The cytochrome bc 1 complex, also known as respiratory complex III (CIII), in the electron-transfer chain of the inner mitochondrial membrane is a homodimer (CIII2) of two biochemically identical protomers. CIII2 catalyses the transfer of electrons from the lipophilic two-electron donor ubiquinol (QH2) to the water-soluble, one-electron acceptor protein cytochrome c, contributing to an electrochemical proton gradient across the membrane. Electron transfer within the complex occurs through the prosthetic groups of the three catalytic core subunits: heme b L and heme b H of cytochrome b (cyt b), heme c 1 of cytochrome c 1 (cyt c 1) and the [2Fe–2S] cluster of the iron–sulfur protein (ISP), often called the Rieske protein after its discoverer. The Rieske domain is tethered to the complex by one transmembrane helix and a connecting flexible linker that acts as a hinge.

(ix) +DQ+NaAsc: reduced by ascorbate and DQ. When DQ and ascorbate were added after purification (+DQ+NaAsc) density in the Qo site increased, indicating a possible low occupancy of DQ in the Qo site. The additional density was in a position similar to atovaquone. The Rieske domain was in a position in which Tyr279 and Cys189 were further apart (3.7 Å) and His190 was closer to Tyr279 (3.4 Å) compared with the ascorbate-reduced sample without added DQ. His190 was ∼2.7 Å away from the DQ density in the Qo site. The Fe–S cluster-bearing tip of the Rieske domain was well-resolved in the two ascorbate-reduced samples. Density at the hinge, where the transition from helix to random coil occurs with Pf-type inhibitors bound, and density distal to the tip was weak, indicating heterogeneity in these regions. In CIII2 with a reduced high-potential chain there was also a clear increase in density for bound quinone in Qo when DQ was added. Addition of the substrate analogue decylubiquinone to CIII2 with a reduced high-potential chain increased the occupancy of the Qo site. Under conditions that favour the enzyme–product complex we observe better density for a quinone substrate in the Qo site, which has been difficult using crystallographic studies.

>MNSLLRLPALKRGVFTMSKRGLATTVSPKTRTSNLKNGLTIASESNPLVQTATVGVWIDAGSRNENAYNNGTAHFFEHLAFKGTDKRSQHQLELDIENMGGHLNAYTSRESTVYYAKSFKDDVPKSVEILADILQHSKLAESAIDREREVITRELEEVNKQYEEVVFDHLHATAFMNQPLGRTILGPRENIQTITNTELRKFITENYTADRMVLVGAGAVDHDALVELAEKYFSHLPSSQSPVPLGTPRSSGEDANQNPIPNFVGSEVRLRDDTMPVAHIAIAVEGVSWTSEDYYTALVAQAIIGNYDRAVGTSRHQGSRLSNIVSENNLANSFQSFSTSYSDTGLWGIYLTSENTTQIDDLVHFTLKEWNRLSTSVSNLQVERAKSQLKAGLLLSLDGTTYVAEDIGRQLTTLGRRVTPAEVEAKLEAVTEHDVRAWAQKTLYDKDIALVGLGPIEGLYDYNRIRNDMSMMRW[2x];>[2x]MTRGVPRLAVAARHFSTAEAAGVKVAAQDGQSPISDLSVVLRGGSRYATVPGVSHILEKFAFQNTVPKSALRFVRELELFGGKLYTHTTREHIVLRTQFLKQDLPYFVDAFANVLKETKFQQFELTERVAPVAELDLLKRESDPAFTALEAAHEVAFRTGLGNSVYAQGYSPVTLEDVKEFARQVYAKQNVAVVGNNVVPADLQQLVGTAFADLQEGSKVTQAGTTTLHGGEARVRTSTGNALTIALPIAEPKPVYHALASFLGGPASMPWSVGASPLAQATVGTHTSVKATYHNYGDAGLFAITIKGDSPAEISQVAHKAVQALKDTGAEVTEEQAARAYAKSKFAAAEAFENPDSSASVIGMELLSGVSRIAPENVQKFTPAELSEAAAQLSASAKPVVAAVGQVHALPFADELF;>MALRKKNSLLNMANSYVLDSPQPSNLNYFWNFGSLLALCLVIQLATGITLAMHYTSHASLAFDSVEHIMRDVNFGWFIRYAHANTASFFFICIYAHMGRNIYYGSYKTPRVLPWSIGVIIFLLLIITAFMGYVLVFGQMSLWGATVICNLVSAIPWLGEDIVHFLWGGFSVGNPTLQRFFALHYLMPFVLAVFALLHLIALHTAGSSNPLGITSNVDKLSMHPYYSFKDLITVFAFLLMFTLFVFFSPDKLGHPDNYIPANPMVTPASIVPEWYLLPFYAILRAIPDKLGGVIAMVAAILILLILPIVDRSIIRGNAFKPISKLLFGFFICNFLLLGVLGQVHIEPPFIVLGQICTIFYFSYFLILLPMVSTIENIFFYIGSLRK[2x];>MRRRRIGVWPENRRVSRLWVSLSPRSCVTCPVPTNQNPPINNHHTPILTQMFKAIPLRQALLGISSAVCAGATTTYYYTTKAEAMTAAEHGLHPAEYPWPQNGMLSTFDHASLRRGYQVYKEVCAACHSLDRIAWRNLVGVTHTTDEAKAFAEELEYDDEPDDEGNPRKRPGKLADYIPGPYPNEQAARAANQGALPPDLSLIAKARHGGADYIFALLTGYPDEPPAGVVLAPGMNYNPYFPGGGIGMARTLFDGVVEYEDGTPATTSQMAKDVAAFLTWAAEPEHDERKKLGLKAIIVISAMLGLSVYIKKFKWSPIKNRKFIYNPPKN[2x];>MSLLRTAAQAVKAPKAYTPLVAAKAFAQTRSVSSQPIGGKSTYKIPDFTPYLKKDRNTDANRLFSYFMIGSFGMLSAAGAKATVQDFLSNMSASADVLAMAKVEVKLGAIPLGKNVIIKWRGKPIFIRHRTSEEIEEANEVNVATLRDPQTDDERVQKPEWLVMIGVCTHLGCVPIGEAGDFGGWFCPCHGSHYDISGRIRRGPAPLNLEIPEYDFADAETLVIG[2x];>[2x]MSYFLTLASEVAESLLPTVAFASEEEKEQDEPVEVESDDDESEEKEDDDEEEDEDDDDDDDDDEVPDPAIALHEAAAEGPCHDFKHHFDECVERVTKAQEAEDYDHAEYKEDCVEEFFHLQHCINDNTADKLFRVLK;>[2x]MASITSVVKTSELILKSPLLSKIVVPLAKTYVKFSGYRQLGFKMNDLIIEETPNMQLALRRLPPTESYDRVYRLIRATQFSLSHKLATGNDITKPEEDDHYLIPYILDVEAEAFEKDALDNLEVVKRK;>MGGNGHYMGWWGHMGSPPQKGIAGYTISPFAARPFAGVVHAAIFNTFRRTKNQALFVILPVSFFYYVWTQASEKNEWLYTKAGRHELAKALAE[2x];>MAWATTFYNVFVKRNSAFVATILASAFVFDMTFETAIDNFWDRINAGKQWKDIRHKYIEAAGDDDEDDE[2x];>MICGEGDYVKKPSYKIVPHFLGFNIPTVSKWIPIFGIWGAAAGIGALFLIEGVPRTRQDILSKIPIIGEHWIREIPASDNPF[2x]>[4x]MGQNMEIDNFLKIERLAENDLPKFIQLIRLFEAVFEMKNFSIPDSEHLQKLLNQNNFYVFVALLENKIVGGLTSYVLEQYYS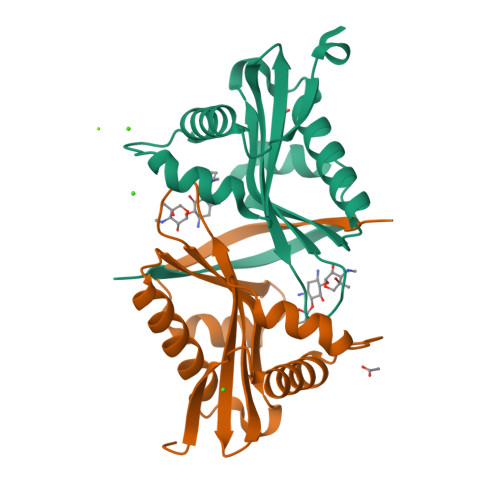EKPLAYIYDLAVDTNWQRQGIGKKLITATNQFYTEKGFEEVFVQADKVDDYALDFARSTKPTAEEQVVHFYYTLK>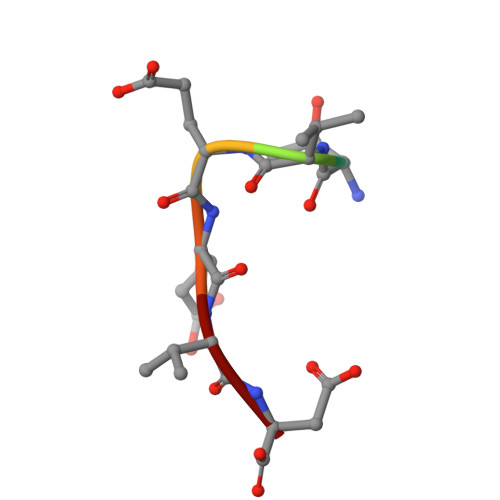 PTVEEVD Group I introns catalyze their own excision from RNA precursors in many organisms through two sequential transesterification reactions. The Tetrahymena thermophila group I self-splicing intron was the first ribozyme to be discovered. To understand how the group I intron promotes catalysis and coordinates self-splicing reactions, we determine the structures of L-16 Tetrahymena ribozyme in complex with a 5′-splice site analog product and a 3′-splice site analog substrate using cryo-EM.

Although S2 has a phosphorothioate substitution at the scissile phosphate to slow down the reaction, it is a racemic mixture of both stereoisomers of the phosphorothioate, one of which slows down the reaction rate by a factor of >10,000 and the other by about 1419, therefore it is very likely that a fraction of complexes containing the latter stereoisomer has catalyzed the chemical step, leading to the Tetrahymena ribozyme Con3. Strikingly different from Con2, in Con3 there is a clear break in the cryo-EM density between G(−1)S2 and u(+1)S2 and continuous density between u(−1)S1 and u(+1)S2, where a new phosphodiester bond should be formed. This supports the conclusion that Con3 has accomplished the second transesterification reaction, which leads to the exon ligation without major conformational changes compared to Con2. In this conformation, the densities for S2-P7 interactions remain resolved, and the densities for the P7ext base pairs also appear at a lower threshold. Notably, some extra density appears at the end of P10 at a lower threshold in Con3, which may be due to the flexibility of the P10 helix, favoring the detachment of the duplex from the active site. The P10 flexibility could be caused by the lack of tertiary contacts holding the P10 helix to the ribozyme active site after its breakage with 5′UCGS2. As the reaction progresses, the ribozyme forms a stable intermediate conformation (Con3), where the exons are ligated, the metal-exon coordination remains but weakens, and the tertiary interactions between 3′-exon and intron are lost. Here, we offer a potential explanation: some extra density can be seen near the end of P10 in Con3, which may be a result of the P10 helix flexibility, favoring the duplex separation from the active site. P10 flexibility may be caused by the lack of tertiary contacts holding the duplex to the ribozyme active site after its breakage with 5′UCGS2, which anchors P10 in the active site via base-pairing interactions (P7ext) to the ribozyme core. Loss of the covalent connection to the duplex P7ext may promote this Con3-Con4 transition.

> UCG;> CCCUCUUAACC;> GGUUUGGAGGGAAAAGUUAUCAGGCAUGCACCUGGUAGCUAGUCUUUAAACCAAUAGAUUGCAUCGGUUUAAAAGGCAAGACCGUCAAAUUGCGGGAAAGGGGUCAACAGCCGUUCAGUACCAAGUCUCAGGGGAAACUUUGAGAUGGCCUUGCAAAGGGUAUGGUAAUAAGCUGACGGACAUGGUCCUAACCACGCAGCCAAGUCCUAAGUCAACAGAUCUUCUGUUGAUAUGGAUGCAGUUCACAGACUAAAUGUCGGUCGGGGAAGAUGUAUUCUUCUCAUAAGAUAUAGUCGGACCUCUCCUUAAUGGGAGCUAGCGGAUGAAGUGAUGCAACACUGGAGCCGCUGGGAACUAAUUUGUAUGCGAAAGUAUAUUGAUUAGUUUUGGAGU> GPHMTDKSDRTDWVALMRAIRDHRDEAAFAELFQHFAPKVKGFLMKSGSVASQAEECAQDVMATVWQKAHLFDPSRASVATWIFTIARNRRIDGLRKDRQPEPEDLFWGPDSEPDQADVYEMQQENARLGRAIARLPEAQRALIERAFFG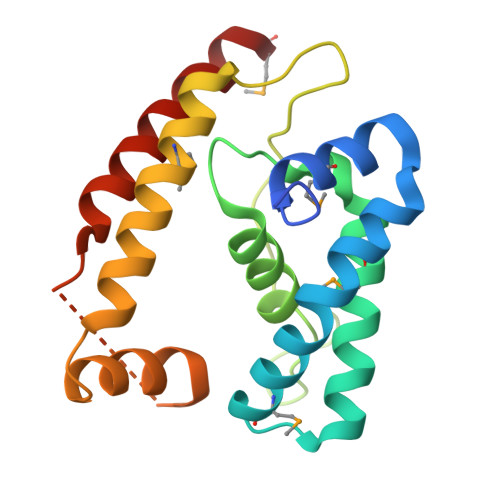DLTHRELAAETGLPLGTIKSRIRLALDRLRQHMS>GSHMKTSYDDTRQHLLDTGYRIMAVKGFSGVGLNEILQSAGVPKGSFYHYFKSKEQFGQALLEDYFRVYLADMDQRFSAPGLNARERLMSYWQKWLDNACPPCDEQRCLVVKLSAEVADLSESMRITLRDGSDGIIERLVGCLGQGRDDGSLAPCDARHMASALYQLWLGASLLS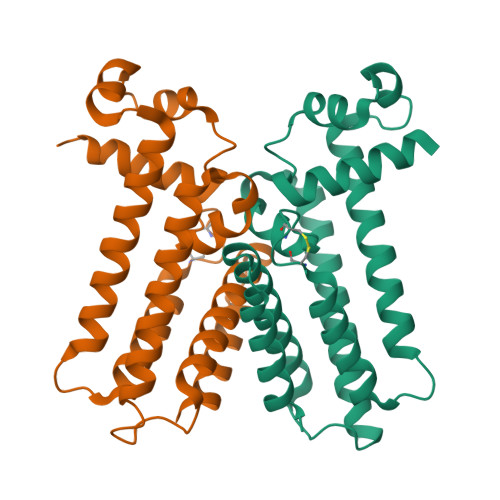KLHRSPGPLETAMQTTRSLLEI[2x]> SMSGASSAVGGSTRSPSPVDPKRGAVQPRYFITTSLTEKERNSVMEAIQKLGQRAVLVDNKVDEILPLNTTHIVLRGPPRSVKALCGVVSSKWLVQPSYVFDSLGAGFWLDEEVEGGLRYFPPPLRCQRFLLTMPEGVVKTMLQRVVEFGGGEVVGTKRNG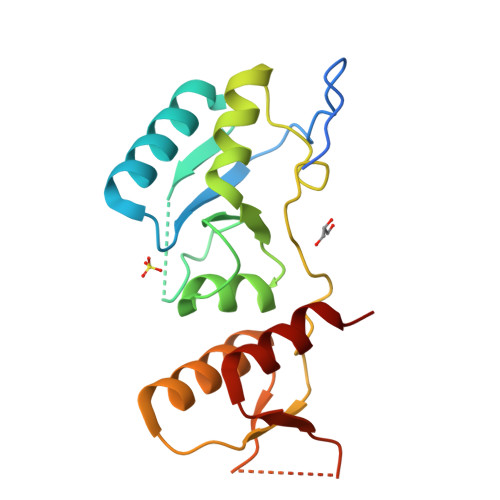SSNDQDVVVVSSGDELLRFAISRD> 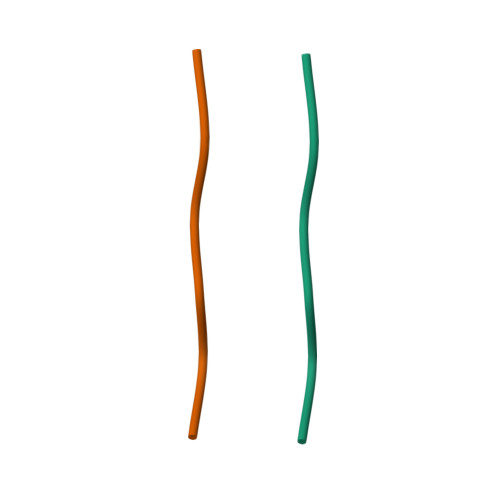SNQNNF> SNRKTSCPIKINQFEGHFMKLQADSNYLLSKEYEELKDVGRNQSCDIALLPENRGKNRYNNILPYDATRVKLSGGSDYINASYIPGNNFRREYIVTQGPLPGTKDDFWKMVWEQNVHNIVMVTQCVEKGRVKCDHYWPADQDSLYYGDLILQMLSESV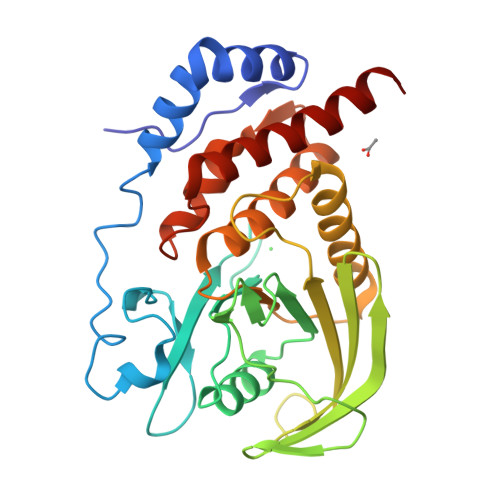LPEWTIREFKICGEEQLDAHRLIRHFHYTVWPDHGVPETTQSLIQFVRTVRDYINRSPGAGPTVVHCSAGVGRTGTFIALDRILQQLDSKDSVDIYGAVHDLRLHRVHMVQTECQYVYLHQCVRDVLRARKLR Rab23 is a member of the Rab family of small GTPases. It plays crucial roles in Hedgehog signaling, ciliary transport, and embryonic development. As a member of the Rab GTPase family, Rab23 acts as a molecular switch by cycling between the GDP-bound inactivated (OFF) state and the GTP-bound activated (ON) state. The structures of the hRab23 in complex with GDP or GMPPNP revealed a typical small GTPase fold of the Ras and Rab family proteins, containing six β-strands and five α-helices.

Like the WT hRab23 protein, the Y79del mutant of hRab237-172 copurified with GDP, as evidenced by clear observation of the electron density of GDP. This observation suggests that the Y79 deletion does not abolish GDP binding. The switch I loop of the hRab237-172 Y79del-GDP structure adopted an opened conformation, similar to that in the WT hRab237-172-GDP structure. The switch II region of the GDP-bound hRab237-172 Y79del, however, exhibited a different conformation relative to that of the WT hRab237-172-GDP structure. The switch II region of the hRab237-172 Y79del mutant was more ordered than that of the WT Rab237-172 structure. The partially disordered region (residues 67–70) observed in the WT hRab237-172-GDP structure formed a 310 helix in the hRab237-172 Y79del mutant structure. However, in the hRab237-172 Y79del-GDP structure, the residues corresponding to the α2 helix in WT hRab237-172 formed a random coil instead of an α-helix, suggesting that the loss of Tyr79 potentially disrupts the secondary structure of the said region. On closer inspection of the mutation site, the loss of Tyr79 resulted in Tyr78 being repositioned to take the place of Tyr79 in the hydrophobic pocket while neighboring Ala77 moved to the original (WT) position of Tyr78. Notably, the occupation of Ala77 in the original position of Tyr78, which is a residue in the hydrophobic triad, potentially altered the interaction surface with binding partners. However, the hRab237-172 Y79del mutant in the presence of Intu–Fuz did not show a significant decrease in luminescence signals (78.2 ± 2.4% relative to buffer control) compared to hRab237-172 Y79del alone (83.5 ± 11.5% relative to buffer control). This observation suggests that the GEF-stimulated nucleotide exchange activity of the hRab237-172 Y79del mutant is impaired.

> SEVAIKMVVVGNGAVGKSSMIQRYCKGIFTKDYKKTIGVDFLERQIQVNDEDVRLMLWDTAGQEEFDAITKAYRGAQACVLVFSTTDRESFEAVSSWREKVVAEVGDIPTVLVQNKIDLLDDSCIKNEEAEALAKRLKLRFYRTSVKEDLNVNEVFKYLAEKYLQK> MAAQGPSPIPTNRLKQIAADACNDAIGSAEFYDHAKTEQWNHQIINTILKAVIAESQPSDSTTPPQFKFAVNSTIVQHLVPSSKLNKPAGGADDKPASTATSTDGKPHVGRRGMHS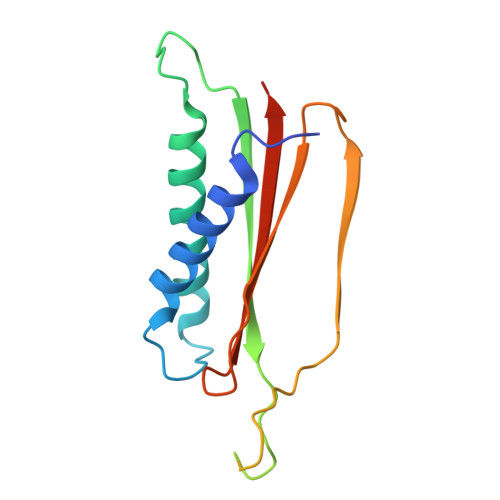ATGAFWNDKTDGMWTYKHEGDESKGMDVVVMLIWIAVLEHHHHHH> MRGSHHHHHHGSMDKDCEMKRTTLDSPLGKLELSGCEQGLHEIKLLGKGTSAADAVEVPAPAAVLGGPEPLMQCTAWL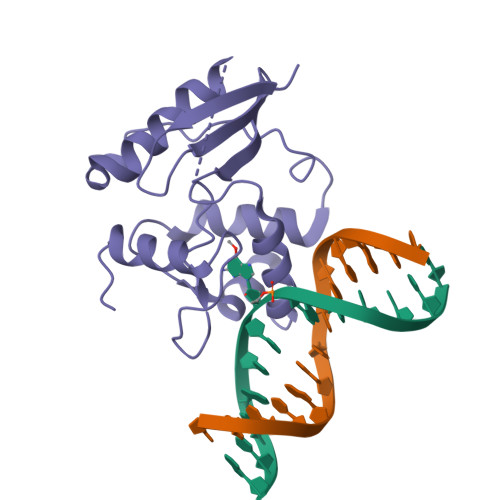NAYFHQPEAIEEFPVPALHHPVFQQESFTRQVLWKLLKVVKFGEVISYQQLAALAGNPKAARAVGGAMRGNPVPILIPSHRVVCSSGAVGNYSGGLAVKEWLLAHEGHRL(2~{R})-~{N}-[5-(5-azanylpyridin-3-yl)-4-ethanoyl-1,3-thiazol-2-yl]-2-carbamimidamido-propanamide 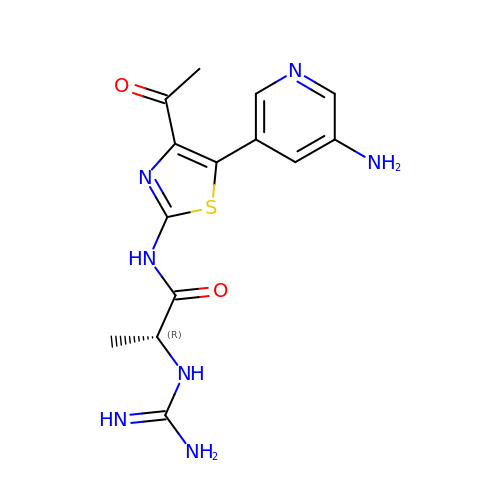| C14 H17 N7 O2 S | GSSILESOVFXWIC-ZCFIWIBFSA-N>GAGAYAYKTIKEDQKRYNERVMGLGLSPEEKQRRAIASATEGGSVPQIRAPSHVPFLLIGGGTAAFAAARSIRARDPGARVLIVSEDPELPYMRPPLSKELWFSDDPNVTKTLQFRQWNGKERSIYFQPPSFYVSAQDLPNIENGGVAVLTGKKVVHLDVRGNMVKLNDGSQITFEKCLIATGGTPRSLSAIDRAGAEVKSRTTLFRKIGDFRALEKISREVKSITVIGEGFLGSELACALGRKSQASGIEVIQLFPEKGNMGKILPQYLSNWTMEKVKREGVKVMPNAIVQSVGVSGGRLLIKLKDGRKVETDHIVTAVGLEPNVELAKTGGLEIDSDFGGFRVNAELQARSNIWVAGDAACFYDIKLGRRRVEHHDHAVVSGRLAGENMTGAAKPYWHQSMFWSDLGPDVGYEAIGLVDSSLPTVGVFAKATAQDNPKSATEQSGT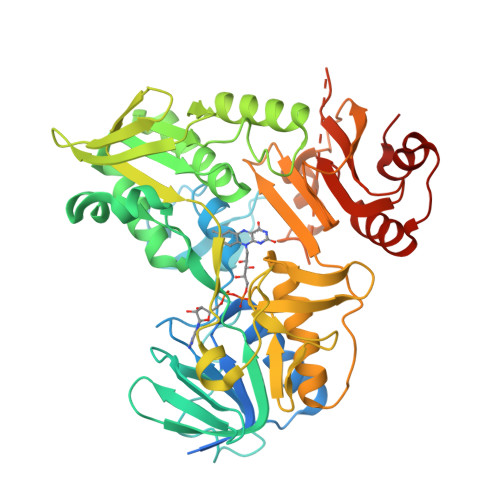GIRSESETESEASEITIPPSAPAVPQVPVEGEDYGKGVIFYLRDKVVVGIVLWNVFNRMPIARKIIKDGEQHEDLNEVAKLFNIHED[2x]4-[4-(2-methylpropyl)-1,2,3-triazol-1-yl]-~{N}-[3,3,3-tris(fluoranyl)propyl]benzamide | C16 H19 F3 N4 O | 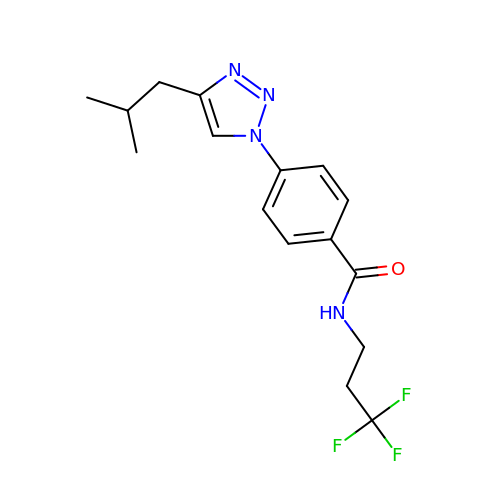LBCXJROJUODEIN-UHFFFAOYSA-N To combat these defenses, Anopheles mosquitoes produce inhibitors belonging to the SG7 protein family that block complement at the alternative C3 convertase, C3bBb. Crystal structures of albicin and SG7.AF reveal a novel four-helix bundle arrangement that is stabilized by an N-terminal hydrogen bonding network. In this study, we describe the structures of albicin and its orthologs SG7.AF (from An. freeborni) and anophensin (from An. stephensi), characterize the binding and mechanism of AP inhibition by these inhibitors, and determine a role for properdin in modulating the inhibitory activity of SG7.AF. SG7 family members are quite similar to one another structurally, but amino acid sequence divergence suggests that specific side chain interactions are key determinants for the observed differences in target affinity.

Previously, we isolated albicin, a member of the salivary SG7 protein family from females of the malaria mosquito An. albimanus, which inhibits activation of the AP in human serum as measured by lysis of rabbit erythrocytes, blocks the cleavage of C3 and factor B in serum, and binds specifically to the C3bBb complex. The structure of albicin consists of a bundle of four α helices stabilized by two disulfide bonds. Helix α1 extends from the N-terminus to Thr 14 and is followed by a section of random coil that extends to Lys 22. The loop connecting helices α3 and α4 extends from Ser 78 to Ser 88, with α4 extending from Val 89 to the C-terminus. The two disulfide bonds link α3 and α4 with Cys 58 forming a disulfide with Cys 113 and Cys 81 linking with Cys 91. The N-terminal amino group of albicin participates in numerous intramolecular electrostatic interactions that appear to be important in stabilizing the overall structure, including three hydrogen bonds with residues forming the turn linking α2 and α3. The carbonyl groups of Val 45, Gly 46, and Tyr 48 form hydrogen bonds with the N-terminal amino group as does ND1 of the imidazole group of His 4 in α1. These interactions may be important for the positioning of the helical elements and stabilization of the helical bundle. The SCIN family structure consists of a bundle of three antiparallel α helices with a long dimension of ∼41 Å and an orthogonal short dimension of ∼14 Å, while the four-helix bundle of albicin has dimensions of 50 and 21 Å. We assessed the oligomeric state of the albicin-inhibited complex observed in SPR experiments using gel filtration chromatography after coincubation of C3b, factor B, and factor D in the presence and absence of albicin and nickel ion, which is known to enhance the binding of C3b with factor B. Albicin markedly reduced the retention volume for complex elution, indicating an increased molecular mass for the inhibited complex beyond that attributable to addition of the inhibitor alone.

>ANNHIRTVLKLFRTIDLDDSKKSFYLTAAKYGIQTQLREPIIRIVGGYLPSTKLSEACVKNMISEVYEIEGDFYSKFSYACEDHAPYSVECLEDARDDYLTQLVELFKETKKCLRE[3x]>[4x]TIPDAMIVIDGHGIIQLFSTAAERLFGWSE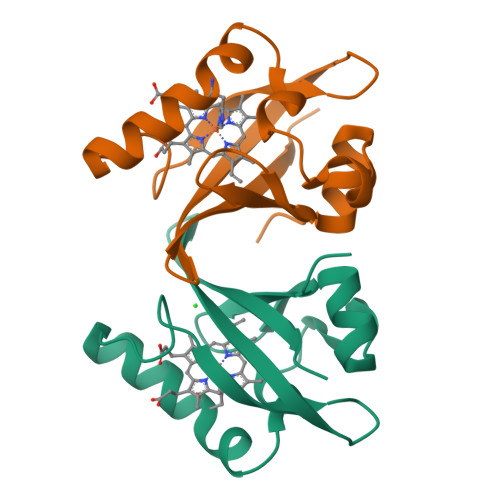LEAIGQNVNILMPEPDRSRHDSYISRYRTTSDPHIIGIGRIVTGKRRDGTTFPMHLSIGEMQSGGEPYFTGFVRDLTEHQQTQARLQEL>[8x]SKPVVRVTQGVLQGSWKVSTHGRTYASFEGVPYARPPVGKYRFREPQHLKPWAGVWDASKTLPQCLQWDPFQQEVSGSENCLYINVHTPKLSAGASLPVVVFIHGGAFMYGAGSLYDVSHLMDRDVVAVTFNYRLGPLGFLSTGDESAPGNAGLKDQAFALQWVKNNVMMFGGNPDSVTLTGCSAGGASVHYHYLSPLSKGNFARGIAFSGAAFASWTHAVKPLQNARSLAAIVGCPTGTNRELVDCLKYRPAEVVVGAQIEMLEFPYQQMFTPFTPTVEPQGTRDAFLTQYPFLVAQAGGMHKVPLITSVTSEEGLYPAAVYQKSPDTLAYLEANWDQLASNIFEYNDTLPVNQRAGVAAKIKQRYLGNKPVSQETYPQLVQALGDRLFAVDVGKLAQIHARHSGQPTYLYRYSFRGEKSLSNMMASNDKNYGVSHADDIFHIFK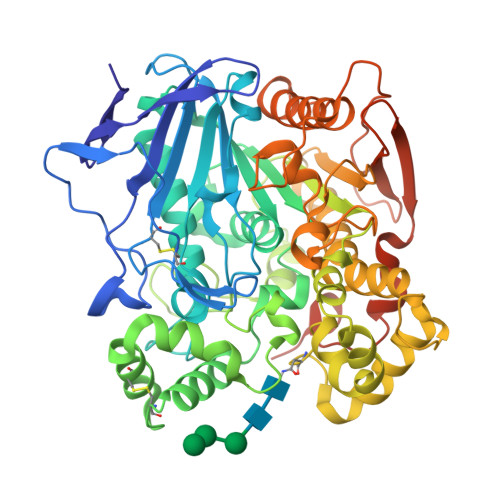FPSLSSTSSEDVRMTEALIDMIYSFSTTGNPKLTNEAPVWTPVTPGSAELSYLEIASPSRMEMKSSSDFGHRSFWDSLGFVENENYRHIRDELENLYFQGHHHHHHHHHH>GEQEDKVSGEKTLAVVSASSDDRPSTRGIINDNTYALGVFRTTANTYAPLYNVKHIYSGGEWGADDVIKVDYRNASFFAYYPYHTATGNYAGLAGGTTLTLQAQLFNAGEDICYGAGEASGGGPVSVYNPFVEFLNMKHAYARLRLTLTRGEKFDKTKKCNIQNITFKSNNANFYLTRSLDIASTAGATGGSAVAAGYVHNPNVNIATGKSVTYEYMFPPQPLDGSKLTILVTVDGVTRSCDISTLGSSLDSGKYYG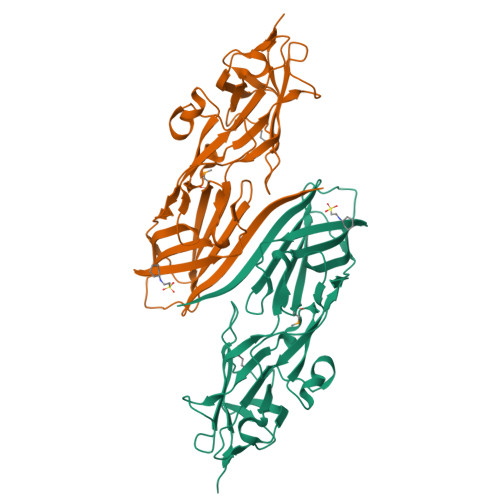VSLTFTDVGIILSSAVVTVNNFGGQGNTQVDTEL[2x]>[2x]MSQNQVPKWIQLNNEIMIQKDGKFQFDKDKEAVHSYFVDYINQNTVFFHNLKEKLDYLVENQYYEEEFLSLYSFEDIKEVFKTAYAKKFRFPSFMSAFKFYNDYALKTNDKKKILERYEDRISIVALFFANGDTEKAKEYVNLMINQEYQPSTPTFLNAGRKRRGELVSCFLLEVNDSLNDISRAIDISMQLSKLGGGVSLNLSKLRAKGEAIKDVENATKGVVGVMKLLDNAFRYADQMGQRQGSGAAYLNIFHRDINDFLDTKKISADEDVRVKTLSIGVVIPDKFVELAREDKAAYVFYPHTIYKEYGQHMDEMDMNEMYDKFVDNPRVKKEKINPRKLLEKL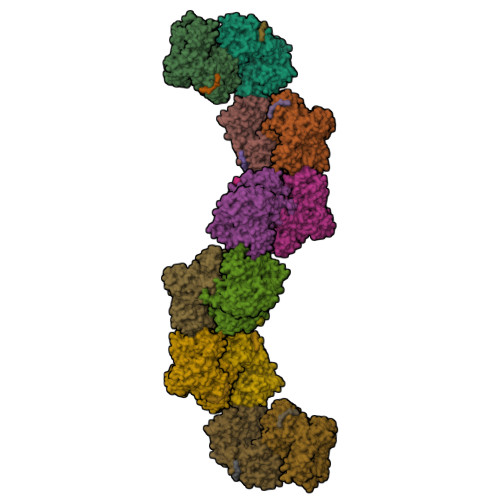AMLRSESGYPYIMFQDNVNKVHANNHISKVKFSNLCSEVLQASQVSSYTDYDEEDEIGLDISCNLGSLNILNVMEHKSIEKTVKLATDSLTHVSETTDIRNAPAVRRANKAMKSIGLGAMNLHGYLAQNGIAYESPEARDFANTFFMMVNFYSIQRSAEIAKEKGETFDQYEGSTYATGEYFDKYVSTDFSPKYEKIANLFEGMHIPTTEDWKKLKAFVAEHGMYHSYRLCIAPTGSISYVQSSTASVMPIMERIEERTYGNSKTYYPMPGLASNNWFFYKEAYDMDMFKVVDMIATIQQHIDQGISFTLFLKDTMTTRDLNRIDLYAHHRGIKTIYYARTKDTGQDSCLSCVV> XGELKALA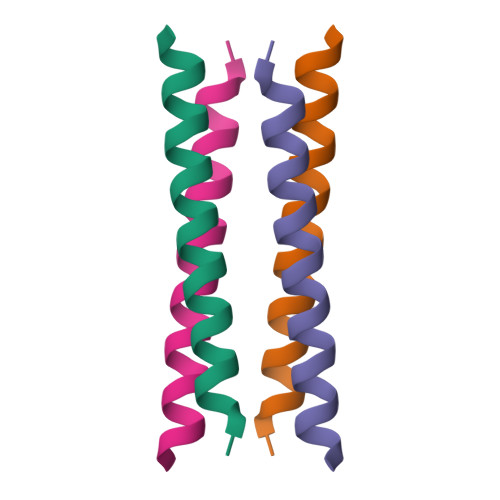QELKALAKELKALAWELKALAKGX(1R,2S,5S)-3-{(2S)-2-(2,3-dihydro-1H-inden-2-yl)-2-[({(1S)-2,2-dimethyl-1-[(2-oxopiperidin-1-yl)methyl]propyl}carbamoyl)amino]acetyl}-6,6-dimethyl-N-{(1S)-1-[oxo(prop-2-en-1-ylamino)acetyl]butyl}-3-azabicyclo[3.1.0]hexane-2-carboxamide 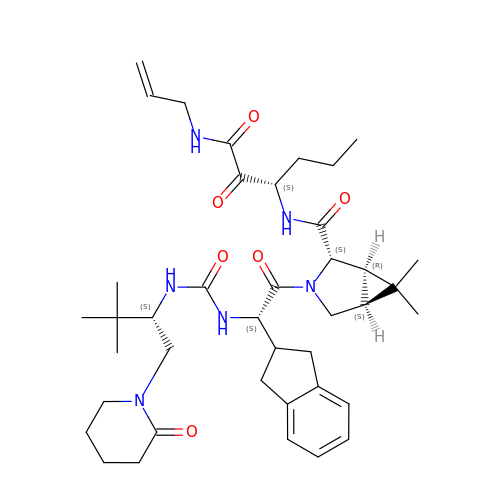| C40 H58 N6 O6 | CRMSMBCBPAEBQR-MUIHSLIFSA-N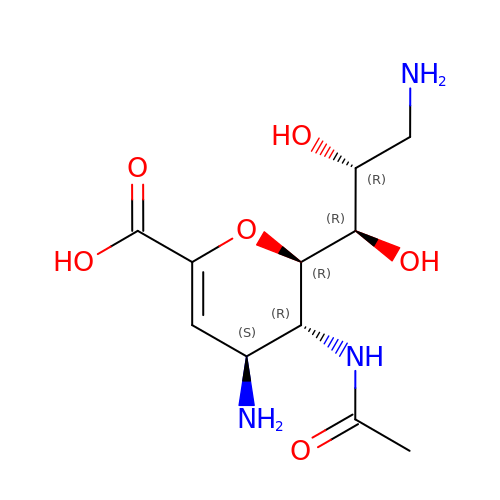4,9-AMINO-2,4-DEOXY-2,3-DEHYDRO-N-ACETYL-NEURAMINIC ACID | C11 H19 N3 O6 | XDWUALXMEIYOQM-UFGQHTETSA-N>[2x]MAEPQPASSGLTDETAFSCCSDPDPSTKDFLLQQTMLRIKDPKKSLDFYTRV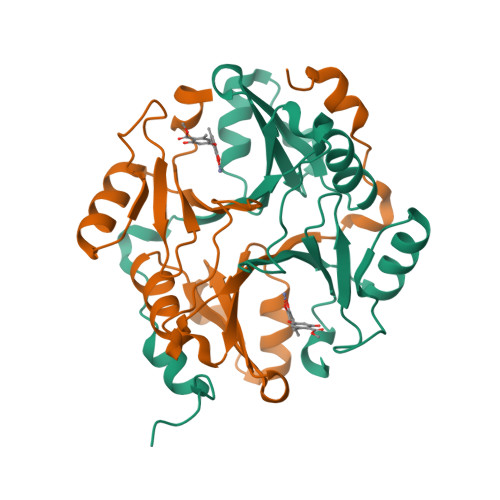LGLTLLQKLDFPAMKFSLYFLAYEDKNDIPKDKSEKTAWTFSRKATLELTHNWGTEDDETQSYHNGNSDPRGFGHIGIAVPDVYSACKRFEELGVKFVKKPDDGKMKGLAFIQDPDGYWIEILNPNKIATII> GAGCAGACGTGA;> CGCCACTCA;> TCAGCG;> TCTGAGTGCGTCTGC

In this work, we exhaustively probe the ability of all 36 immobile HJ sequences to form DNA crystals in two different designed systems. Three separate self-assembling DNA crystal systems are described in this report: the “4 × 5” and “4 × 6” designs (collectively referred to as the 4 × N systems), and a third construct with a “scrambled” sequence variant of the 4 × 6 lattices. Self-assembly was mediated by three constituent oligonucleotides: (S1) containing four sequence repeats of either 5 or 6 bases; (S2) composed of 21 bases containing complementary regions to both (S1); and (S3) which forms the second junction crossover. The HJ serves as the fundamental component at the core of each unit, and the ultimate assembly of the full lattice is facilitated by the complementary 2-base sticky ends that tail each duplex.

Seventeen of the 36 junctions successfully crystallized, a 47% success rate. Unlike the 4 × 5 motif, nearly all of the 4 × 6 junction sequences had a strong preference for crystallization in buffers containing ≥2.0 M salts (e.g., LiCl, Li2SO4, KCl, and NaCl), with the majority preferring slightly basic pH conditions in cacodylic acid. The average cell constants for the P32 crystals were a = b = 68.29 Å c = 55.68 Å. The c-axis, in particular, was ~5 Å shorter, and had a much larger degree of variability (σ = 1.97), than those that crystallized using the 4 × 5 motif. The broad range of the short axis spanned from 52.77 to 60.36 Å, and we posit that the flexible axis lengths could be responsible for rendering a larger number of junctions fatal than the 4 × 5 system. The average junction angles of 54.60° (σ = 1.44) and 58.37° (σ = 2.3) for the P32 and R3 symmetries, respectively, along with their preference for salts or organic solvents, were likely the major contributing factors that yielded the divergent lattices.> SNAEVMEFN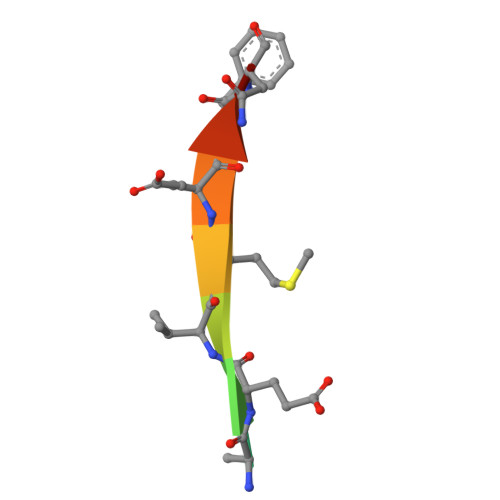P> MANFMIYPISKDLKNGNSELVRVYSKSKEIQYIKIYTKKI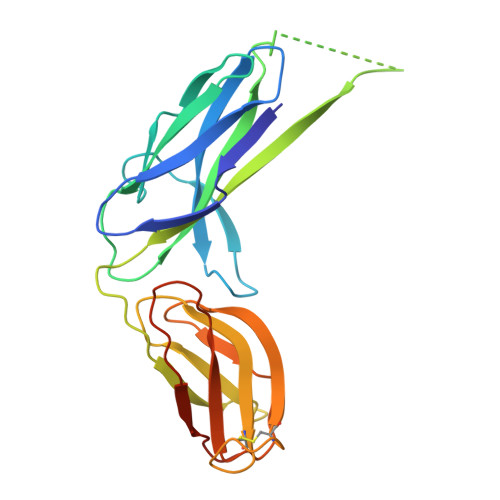INPGTTEEYEVDIPNWDGGLVVTPQKVILPAGASKSIRLTQFKIPKKEEVYRVYFEAVKPDSKENVIDNKKLTIELSVNIIYAALIRSLPSEQNISLNISRNAKKNIIIYNNGNVRAGVKDIYFCKSSNIDDNCVKKAYNKNIYPEKSFDTLVNNNFSYVFIKLNHEGIEKEQGLIQLKVPAAWSHPQFEK>ANPLYQKHIISINDLSRDDLNLVLATAAKLKANPQPELLKHKVIASCFFEASTRTRLSFQTSMHRLGASVVGFSDSANTSLGKKGETLADTISVISTYVDAIVMRHPQEGAARLATEFSGNVPVLNAGDGSNQHPTQTLLDLFTIQQTEGRLDNLHVAMVGDLKYGRTVHSLTQALAKFDGNRFYFIAPDALAMPEYILDMLDEKGIAWSLHSSIEEVMAEVDILYMTRVQKERLDPSEYANVKAQFVLRASDLHNAKANMKVLHPLPRVDEIATDVDKTPHAWYFQQAGNGIFARQALLALVLNRDLVL[2x];>MTHDNKLGVEAIKRGTVIDHIPAQIGFKLLSLFKLTETDQRITIGLNLPSGEMGRKDLIKIENTFLSEDQVDQLALYAPQATVNRIDNYEVVG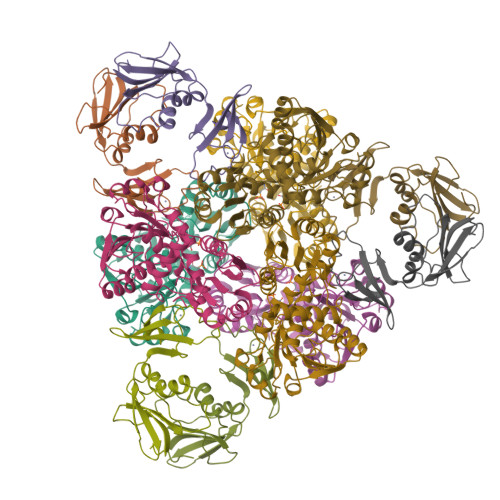KSRPSLPERIDNVLVCPNSNCISHAEPVSSSFAVRKRANDIALKCKYCEKEFSHNVVLAN[2x]Through the COVID-19 pandemic it gained more prominence by being a key pathogen in respiratory co-infections. This study will present a structural analysis of StmPr1, S. maltophilia’s main virulence factor, an excreted serine protease. StmPr1 is a member of the subtilases family defined by Siezen & Leunissen et al.. It shows the main structural and functional elements of the family, such as a reactive triad consisting of Asp42, His105, and Ser28922. The catalytic triad consisting of Asp42, His105, and Ser289 is located on top of β1 (Asp42), α4 (His105), and α10 (Ser289).

To understand the interaction of StmPr1 with inhibitors, we investigated structures of StmPr1 in complex with the well-known protease inhibitor PMSF and the peptide aldehyde inhibitors Leupeptin and Chymostatin, as well as the peptide-like boron-based inhibitor Bortezomib. All inhibitors bind covalently to Ser289, forming a tetrahedral transition state supported by the main chain amid of Ser289 and the sidechain amino group of Asp207. PMSF is further stabilized by a water molecule and Bortezomib is stabilized by the catalytic triad His105. Besides the covalent bond to Ser289, the phenyl part of PMSF is coordinated into the P1 site of the substrate binding cleft. While PMSF shows a IC50 of 125,43 µM needing a concentration of 1 mM to totally eradicate enzymatic activity and Leupeptin even shows a higher IC50 with 130,3 µM, Bortezomib has an IC50 of 1,97 µM, eradicating the activity at 100 µM and Chymostatin has an IC50 of 0,04 µM and needs 10 µM for total inhibition.

> LAPNDPYYQQYQWHLHNATGGINAPSAWDVSQGEGVVVAVLDTGILPQHPDLVGNLLEGYDFISDASTSRRATNDRVPGAQDYGDWVENDNECYTGSVAEDSSWHGTHVAGTVAEQTNNGVGMAGVAHKAKVLPVRVLGKCGGYLSDIADAITWASGGTVAGVPANANPAEVINMSLGGSGSCDGTYQDAINGAISRGTTVVVAAGNETDNASKYRPASCDGVVTVGATRITGGITYYSNYGSRVDLSGPGGGGSVDGNPGGYVWQSGSDAATTPESGSYSYMGMGGTSMASPHVAAVAALVQSALIAAGKDPLAPAAMRTLLKETARPFPVSIPTATPIGTGIVDAKAALASALE> HHHHHHHHMSWLLFLAHRVALAALPCRRGSRGFGMFYAVRRGRKTGVFLTWNECRAQVDRFPAARFKKFATEDEAWAFVRKSASPEVSEGHENQHGQESEAKASKRLREPLDGDGHESAEPYAKHMKPSVEPAPPVSRDTFSYMGDFVV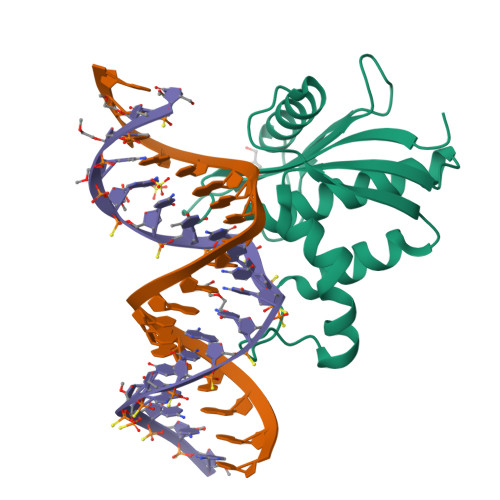VYTDGCCSSNGRRRPRAGIGVYWGPGHPLNVGIRLPGRQTNQRAEIHAACKAIEQAKTQNINKLVLYTNSMFTINGITNWVQGWKKNGWKTSAGKEVINKEDFVALERLTQGMDIQWMHVPGHSGFIGNEEADRLAREGAKQSED6-amino-2-methyl-1,7-dihydro-8H-imidazo[4,5-g]quinazolin-8-one | C10 H9 N5 O 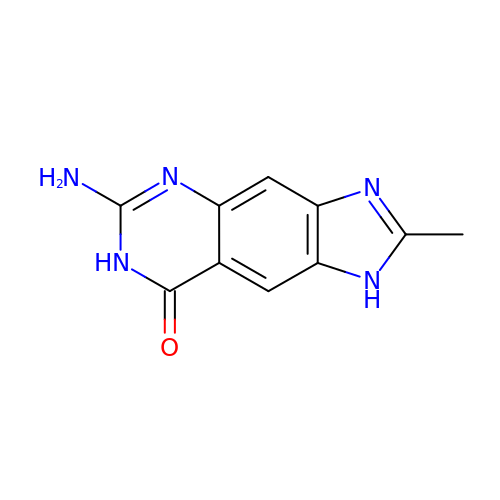| PLJNUNPYZVVIRA-UHFFFAOYSA-N>[12x]XGEIGQALKEIGKALKEIGYALKEIGQALKGX

Here we describe the successful de novo design and structural resolution of a coiled-coil peptide that assembles into multiple, distinct conformational states under the same conditions. The peptide forms an open αHB and a compact α-helical sandwich. We reasoned that introducing glycine (Gly, G) into this sequence should increase structural dynamics and potentially access alternative states, as Gly has the most backbone freedom of any α-amino acid, and it allows close approach of α helices. Therefore, we introduced Gly at all of the e sites to give CC-Type2-(LaIdGe)4.

Next, we crystallised and solved an X-ray structure for a 4-bromophenylalanine variant of CC-Type2-(LaIdGe)4. To our surprise, the asymmetric unit contained two distinct and strikingly different α-helical hexamers: an open, C6-symmetric barrel; and a closed, C2-symmetric sandwich with a consolidated hydrophobic core. To a first approximation, both structures have two three-helix sheets with similar helix–helix interfaces and KIH interactions expected for Type-2 coiled coils. The main difference is that the two α-helical sheets of the open state are related cyclically to give the C6 symmetry; whereas, those of the closed state is sheared perpendicular to the central C6 axis, to give a C2-symmetric bundle. As a result, in the latter, the aliphatic residues form a compact hydrophobic core. However, relative to the open barrel, the remaining chains of the closed state are rearranged significantly with average translations in the paired helices ‘3’, ‘4’, and ‘5’ of 5.92, 6.98, and 6.05 Å, respectively. We propose that the introduction of Gly at e’ in CC-Type2-(LaIdGe)4 perturbs this balance. The lack of side chain allows the helices to pack more closely together. This is apparent on closer examination of the structures: in the open state, the Cα atoms of the Ala-13 residue at g sites of neighbouring helices are spaced regularly at ≈9.3 Å; whereas, in the closed state the average distance is ≈8.8 Å. The helix–helix–helix angles are all ≈120˚ in the open state but vary between 90˚ and 150˚ in the close state.> GVALGATRVIYPAGQKQVQLAVTNNDENSTYLIQSWVENADGVKDGRFIVTPPLFAMKGKKENTLRILDATNNQLPQDRESLFWMNVKAIPSMDKSKLTENTLQLAIISRIKLYYRPAKLALPPDQAAEKLRFRRSA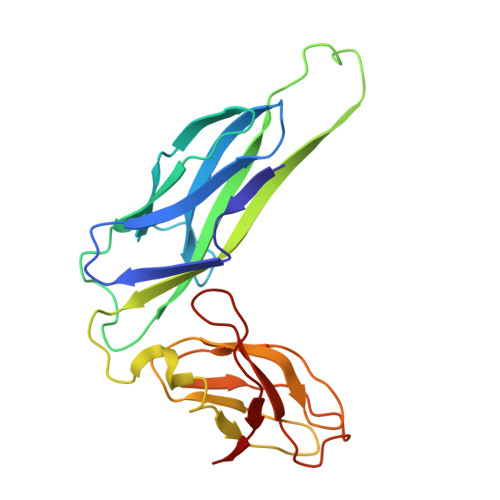NSLTLINPTPYYLTVTELNAGTRVLENALVPPMGESTVKLPSDAGSNITYRTINDYGALTPKMTGVME7-(4-methylpiperazin-1-yl)-N-(5-methyl-1H-pyrazol-3-yl)-2-[(E)-2-phenylethenyl]quinazolin-4-amine 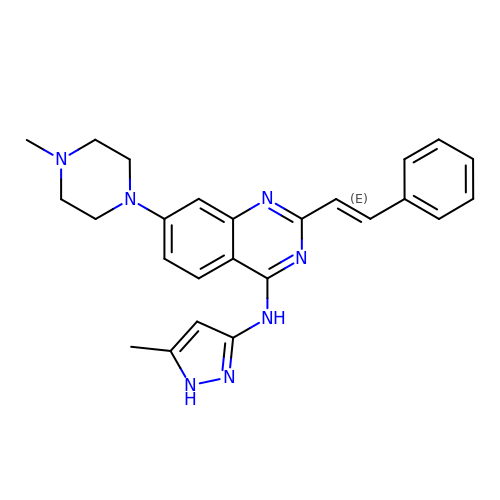| C25 H27 N7 | DKCSQCAVMRLWQW-DHZHZOJOSA-N> MKSSHHHHHHENLYFQSNAETIEIIKDLFEHLCGVRVHRTYEDDTGLWFDTSQGSKNGIMDYKLGFVKSQAENTTEVDTEVIYVPLLKQRTAEELQELQKKLPDYLFETLSFPLRSLNQFYIKMSKSLNKK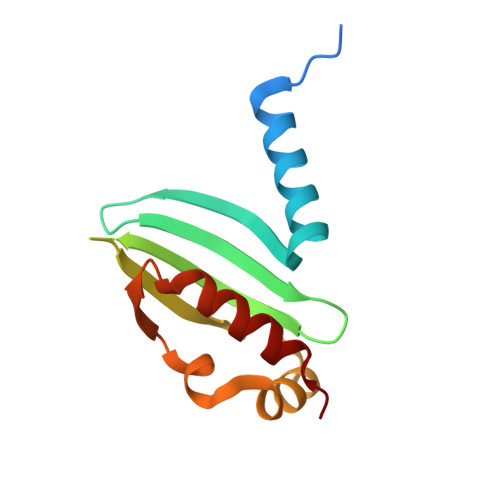V> AEETSFVFSKFKPLEPNLILQGDALVTVAGVLQLTNVDKNGVPEPSSLGRATYSAPINIWDSATGLVASFATSFRFTIYAPNIATIADGLAFFLAPVASAPDSGGGFLGLFDSAVSGSTYQTVAVEFDTYENTVFTDPPY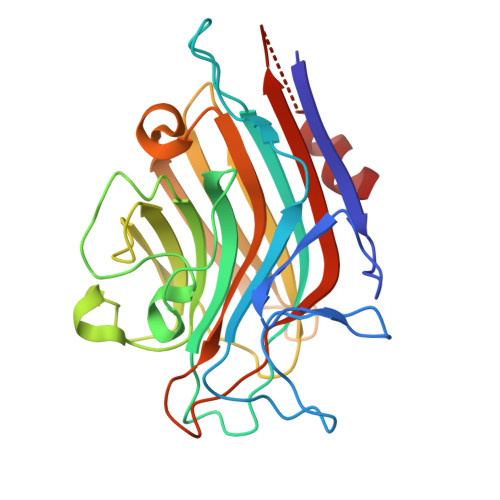THIGFDVNSISSIKTVKWSLANGEAAKVLITYNSAVKLLVASLVYPSSKTSFILADIVDLSSVLPEWVRVGFSAATGASGGKIETHDVFSWSFASKLAGXXTKDSSFLDGG> MDLLKRHLAPIVPDAWSAIDEEAKEIFQGHLAGRKLVDFRGPFGWEYAAVNTGELRPIDDTPEDVDMKLRQVQPLAEVRVPFTLDVTELDSVARGATNPDLDD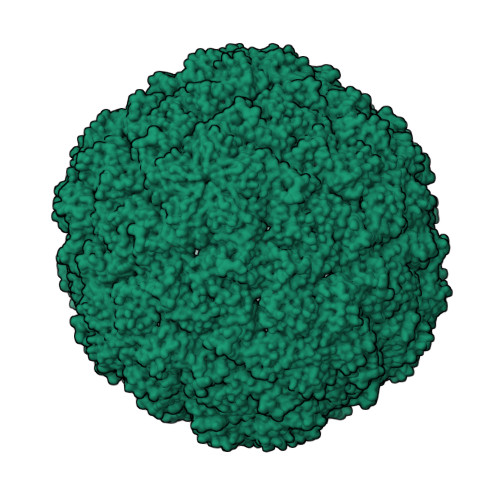VARAAERMVEAEDSAIFHGWAQAGIKGIVDSTPHEALAVASVSDFPRAVLSAADTLRKAGVTGPYALVLGPKAYDDLFAATQDGYPVAKQVQRLVVDGPLVRANALAGALVMSMRGGDYELTVGQDLSIGYAFHDRSKVELFVAESFTFRVLEPGAAVHLRYA> AGGHGDVGMHVKEKEKNKDENKRKDEERNKTQEEHLKEIMKHIVKIEVKGEEAVKKEAAEKLLEKVPSDVLE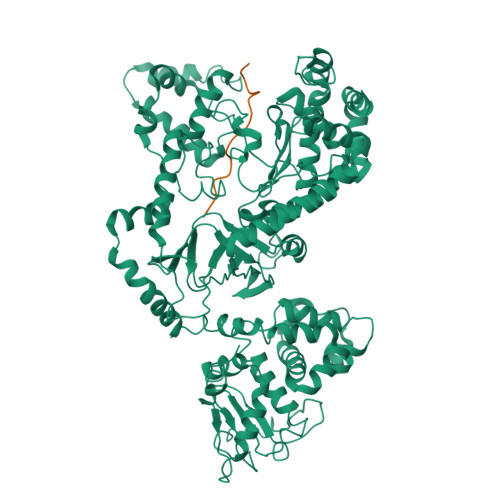MYKAIGGKIYIVDGDITKHISLEALSEDKKKIKDIYGKDALLHEHYVYAKEGYEPVLVIQSSEDYVENTEKALNVYYEIGKILSRDILSKINQPYQKFLDVLNTIKNASDSDGQDLLFTNQLKEHPTDFSVEFLEQNSNEVQEVFAKAFAYYIEPQHRDVLQLYAPEAFNYMDKFNEQEINLSLEELKDQRMLSRYEKWEKIKQHYQHWSDSLSEEGRGLLKKLQIPIEPKKDDIIHSLSQEEKELLKRIQIDSSDFLSTEEKEFLKKLQIDIRDSLSEEEKELLNRIQVDSSNPLSEKEKEFLKKLKLDIQPYDINQRLQDTGGLIDSPSINLDVRKQYKRDIQNIDALLHQSIGSTLYNKIYLYENMNINNLTATLGADLVDSTDNTKINRGIFNEFKKNFKYSISSNYMIVDINERPALDNERLKWRIQLSPDTRAGYLENGKLILQRNIGLEIKDVQIIKQSEKEYIRIDAKVVPKSKIDTKIQEAQLNINQEWNKALGLPKYTKLITFNVHNRYASNIVESAYLILNEWKNNIQSDLIKKVTNYLVDGNGRFVFTDITLPNIAEQYTHQDEIYEQVHSKGLYVPESRSILLHGPSKGVELRNDSEGFIHEFGHAVDDYAGYLLDKNQSDLVTNSKKFIDIFKEEGSNLTSYGRTNEAEFFAEAFRLMHSTDHAERLKVQKNAPKTFQFINDQIKFIINS;> MLARRKPVLPALTINP> SNAMSEQSICQARAAVMVYDDANKKWVPAGGSTGFSRVHIYHHTGNNTFRVVGRKIQDHQVVINCAIPKGLKYNQATQTFHQWRDARQVYGLNFGSKEDANVFASAMMHALEVLGGSGSGFDDFPPPPPPPPVDYEDEEAA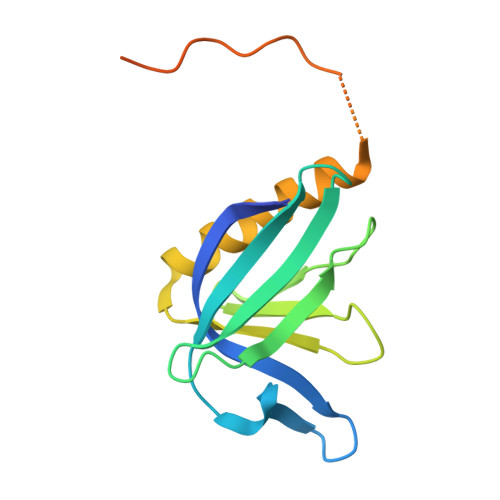VVQYNDPYADGDPAW> MVPISPIETVPVKLKPGMDGPKVKQWPLTEEKIKALVEICTEMEKEGKISKIGPENPYNTPVFVIKKKDSTKWRKLIDLRELNKRTQDFWEVQLGIPHPAGLKKKKSVTVLDVGDAYYSVPLDEDFR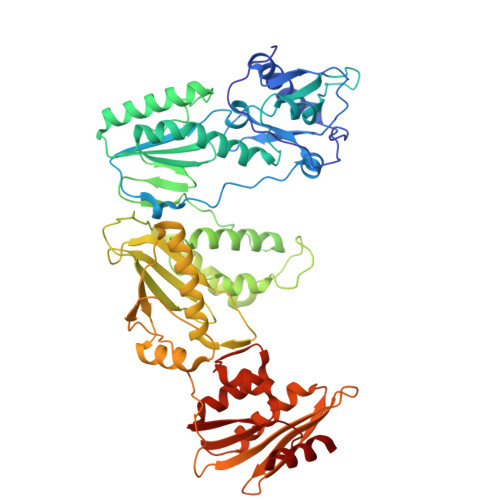KYTAFTIPSINNETPGIRYQYNVLPMGWKGSPAIFQSSMTKILEPFKKQNPDIVIYQYMDDLYVGSDLEIGQHRTKIEELRQHLLRWGLTTPDKKHQKEPPFLWMGYELHPDKWTVQPIVLPEKDSWTVNDICKLVGKLNWASQIYPGIKVRQLSKLLRGTKALTEVIPLTEEAELELAENREILKEPVHGVYYDPSKDLIAEIQKQGQGQWTYQIYQEPFKNLKTGKYARMRGAHTNDVKQLTEAVQKITTESIVIWGKTPKFKLPIQKETWETWWTEYWQATWIPEWEFVNTPPLVKLWYQLEKEPIVGAETFYVDGAANRETKLGKAGYVTNKGRQKVVPLTNTTNQKTELQAIYLALQDSGLEVNIVTNSQYALGIIQAQPDKSESELVNQIIEQLIKKEKVYLAWVPAHKGIGGNEQVDKLVSA> QQKSLTLIVALTTSYGIGRSNSLPWKLKKEISYFSRVTSFVPTFDSFESMNVVLMGRKTWESIPLQNRPLKGRINVVITRNAAAAAAAAIHSAKSLDHALE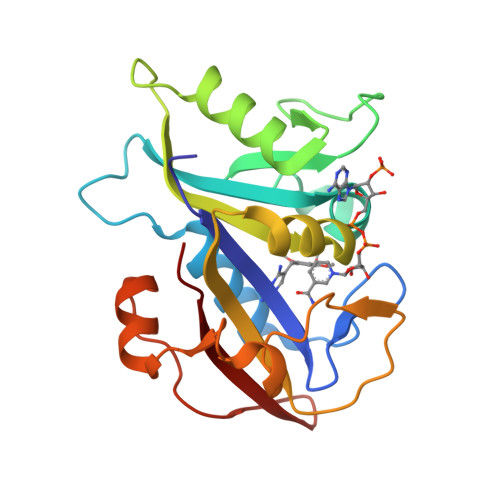LLYRTYGSESSVQINRIFVIGGAQLYKAAMDHPKLDRIMATIIYKDIHCDVFFPLKFRDKEWSSVWKKEKHSDLESWVGTKVPHGKINEDGFDYEFEMWTRDL>[2x]MKKTKIVCTIGPKTESEEMLAKMLDAGMNVMRLNFSHGDYAEHGQRIQNLRNVMSKTGKTAAILLDTKGPEIRTMKLEGGNDVSLKAGQTF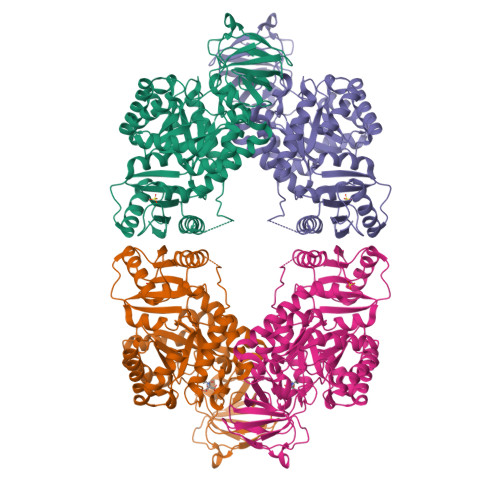TFTTDKSVIGNSEMVAVTYEGFTTDLSVGNTVLVDDGLIGMEVTAIEGNKVICKVLNNGDLGENKGVNLPGVSIALPALAEKDKQDLIFGCEQGVDFVAASFIRKRSDVIEIREHLKAHGGENIHIISKIENQEGLNNFDEILEASDGIMVARGDLGVEIPVEEVIFAQKMMFEKCIRARKVVITATQMLDSMIKNPRPTRAEAGDVANAILDGTDAVMLSGESAKGKYPLEAVSIMATICERTDRVMNSRLEFNNDNRKLRITEAVCRGAVETAEKLDAPLIVVATQGGKSARAVRKYFPDATILALTTNEKTAHQLVLSKGVVPQLVKEITSTDDFYRLGKELALQSGLAHKGDVVVMVSGALVPSGTTNTASVHVL>[2x]MKNRIDPELRAMLDMFPPLNLDDVQATRKAMEEAAQLTEL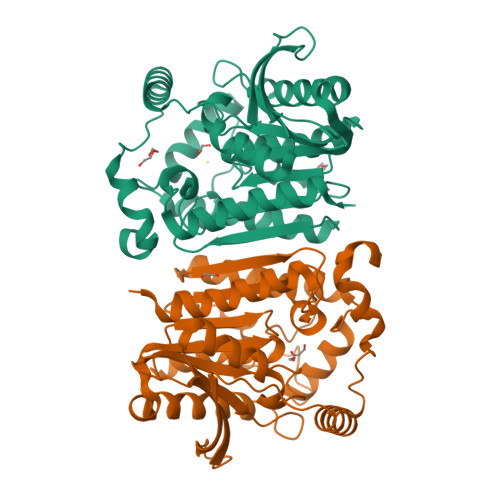PVDEEVVVSNRMVPGPEDNPYVRVRIYEPKEKIEKLPGLLWIHGGGYVLGAPEGDDLLCQRFVKEANCVVVSVDYRLAPEHPYPAPLEDCYAALQWFAKKVDELGVDASRIGVGGQSAGGGLTAALALLARDRKGPELCFQMPLYPMIDDKNNSPSSLEITGNLIWNHDLNEKGWSMYLDGKNGTDDVPVHAAPARATDLTNLPYTYTCVGQLDPFRDETLDYVKRLCQAGVDVEFHLYPGAYHGFETLNPAAAVSQRALAEYVGAVKHVLNREKVVERK> AAA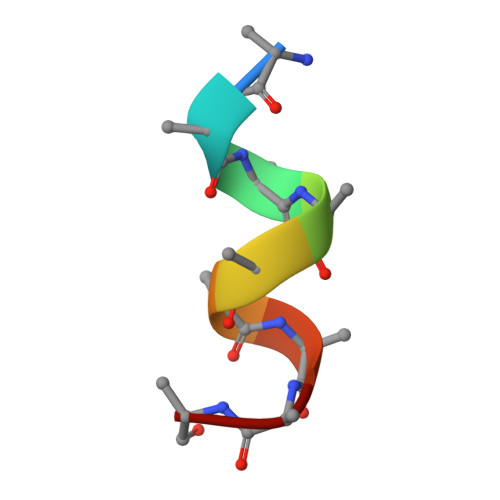AAAAAA>GPLGSGGGTIAMLNEISSDTLEQLYSLAFNQYQSGKYEDAHKVFQALCVLDHYDSRFFLGLGACRQAMGQYDLAIHSYSYGAVMDIKEPRFPFHAAECLLQKGELAEAESGLFLAQELIANKPEFKELSTRVSSMLE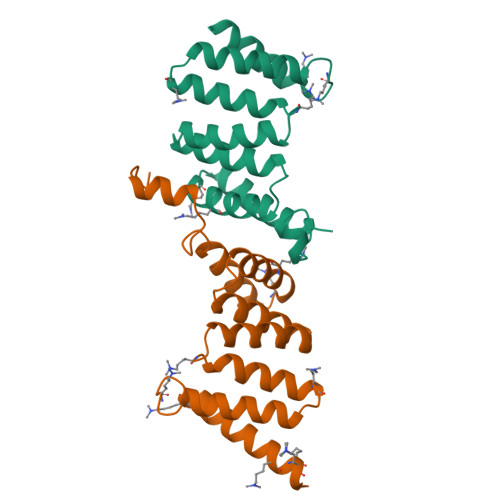AIKLKKEMKHE[2x]> MAQNLPTIALLATGGTIAGSGVDASLGSYKSGELGVKELLKAIPSLNKIARIQGEQVSNIGSQDMNEEIWFKLAQRAQELLDDSRIQGVVITHGTDTLEESAYFLNLVLHSTKPVVLVGAMRNASSLSADGALNLYEAVSVAVNEKSANKGVLVVMDDTIFSVREVVKTHTTHVSTFKALNSGAIGSVYYGKTRYYMQPLRKHTTESEFSLSQLKTPLPKVDIIYTHAGMTPDLFQASLNSHAKGVVIAGVGNGNVSAGFLKAMQEASQMGVVIVRSSRVGSGGVTSGEIDDKAYGFITSDNLNPQKARVL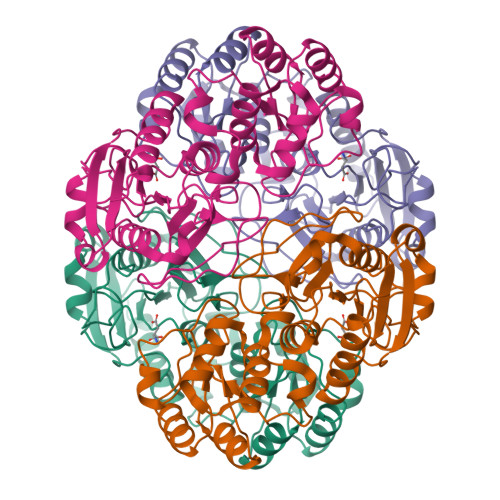LQLALTKTNDKAKIQEMFEEY>[6x]GPLGSSTMGQVGRQLAIIGD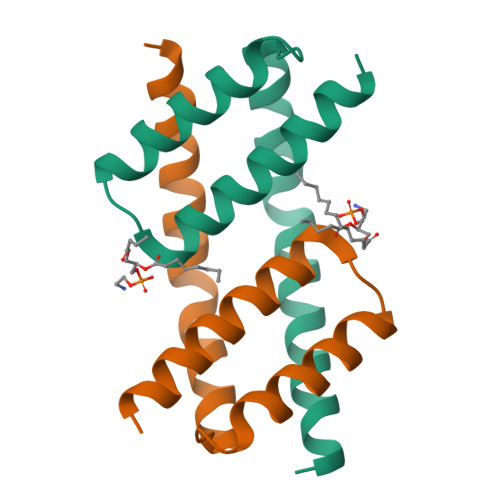DINRRYDSEFQTMLQHLQPTAENAYEYFTKIATSLFESGINWGRVVALLGFGYRLALHVYQHGLT>GAMGGAHKVRAGGPGLERAEAGVPAEFSIWTREAGAGGLAIAVEGPSKAEISFEDRKDGSCGVAYVVQEPGDYEVSVKFNEEHIPDSPFVVPVASPS[2x];>LNWKQDSNPLYKSAITTTINPRFQEADSPTL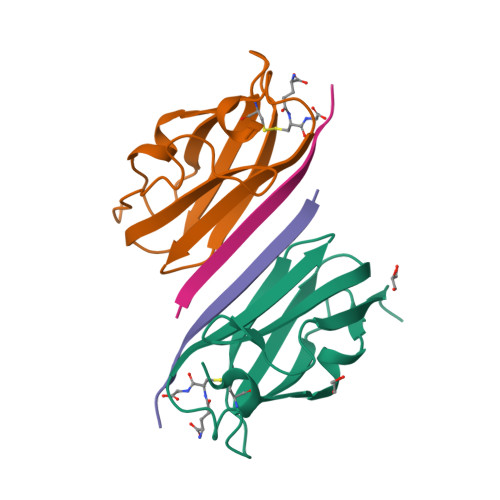[2x]>MEGGGKPNSSSNSRDDGNSVFPAKASATGAGPAAAEKRLGTPPGGGGAGAKEHGNSVCFKVDGGGGGGGGGGGGEEPAGGFEDAEGPRRQYGFMQRQFTSMLQPGVNKFSLRMFGSQKAVEKEQERVKTAGFWIIHPYSDFRFYWDLIMLIMMVGNLVIIPVGITFFTEQTTTPWIIFNVASDTVFLLDLIMNFRTGTVNEDSSEIILDPKVIKMNYLKSWFVVDFISSIPVDYIFLIVEKGMDSEVYKTARALRIVRFTKILSLLRLLRLSRLIRYIHQWEEIFHMTYDLASAVVRIFNLIGMMLLLCHWDGCLQ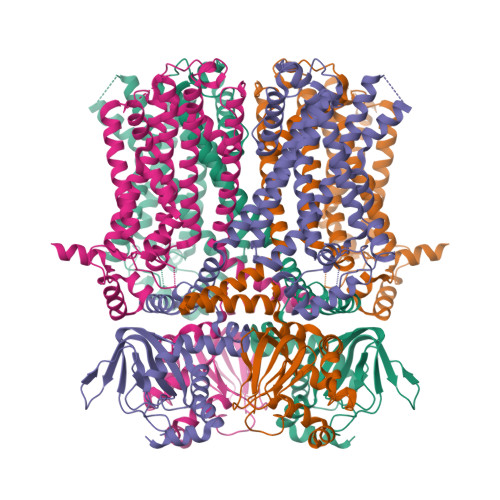FLVPLLQDFPPDCWVSLNEMVNDSWGKQYSYALFKAMSHMLCIGYGAQAPVSMSDLWITMLSMIVGATCYAMFVGHATALIQSLDSSRRQYQEKYKQVEQYMSFHKLPADMRQKIHDYYEHRYQGKIFDEENILNELNDPLREEIVNFNCRKLVATMPLFANADPNFVTAMLSKLRFEVFQPGDYIIREGAVGKKMYFIQHGVAGVITKSSKEMKLTDGSYFGEICLLTKGRRTASVRADTYCRLYSLSVDNFNEVLEEYPMMRRAFETVAIDRLDRIGKKNSILLQKFQKDLNTGVFNNQENEILKQIVKHDREMVQAALPRESSSVLNTDPDAEKPRFASNL[4x]Typical SBP proteins recognize a substrate using two α/β domains, whereas the single-domain substrate-binding protein from Rhodothermus marinus (RmSBP) has a single α/β domain. The crystal structure and flexibility of RmSBP have been established, but its molecular function is unknown. Recently, radiation damage to the selenomethionine-substituted single-domain substrate-binding domain from Rhodothermus marinus (SeMet-RmSBP) was investigated. Global and specific radiation damage from four datasets collected by repeatedly exposing a single RmSBP-SeMet crystal to X-rays were analyzed.

Therefore, the diffraction intensity and radiation damage were not directly comparable, and the diffraction data were collected from a single crystal by rotating it 360°. The diffraction data collected from 1, 2, 3, and 4 X-ray exposures of SeMet-RmSBP crystals were designated Dose I, II, III, and IV, respectively. For the Dose I dataset, images 1–6 were missing. Accordingly, the number of images for Dose I deposited in ZENODO is 354, and the number of images for Dose II, III, and IV was 360. The resolutions of Dose I, II, III, and IV of the structure factor and coordinate deposited in PDB were 1.50, 1.58, 1.68, and 1.75 Å, respectively. Doses I, II, III, and IV were 1.46, 1.56, 1.63, and 1.70 Å, respectively, showing improved resolution compared with the previous report (Doses I, II, III, and IV were 1.50, 1.58, 1.68, and 1.75 Å). As previously reported, with an increase in X-ray exposure, the diffraction limit and I/sigma of SeMet-RmSBP tended to decrease, whereas Rmerge, Rmeas, Rpim, and B-factor tended to increase. As the X-ray exposure time increased, the negative electron density map at the Se atom site of SeMet concomitantly increased; however, a negative density map for other atoms in SeMet was not observed. The results indicate that the Se atom is more sensitive to radiation damage compared with other atoms.

>[2x]PETETEVTPIQQLFLIKELKPGIARIGVIWDKNAANRDEVLPQLQRASAATGIKVVVAEVASLQEVAPQFRTLLRDHQVEALWVLEESGLLGQAAARSFLIKNATQAGMPVFAPSETWLKEGACVTWRKDAEGIRLVVNKAVAEAMGITIPAKYQDRTAFLAMN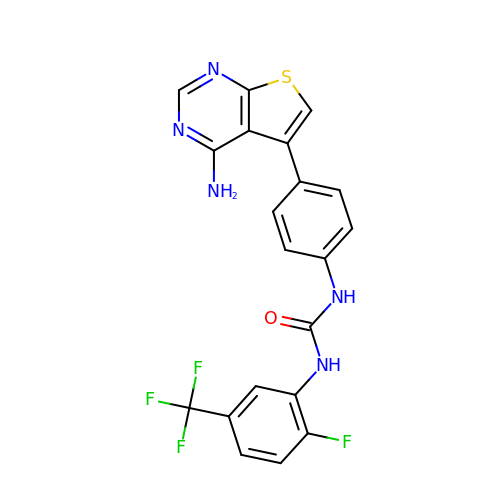1-[4-(4-aminothieno[2,3-d]pyrimidin-5-yl)phenyl]-3-[2-fluoro-5-(trifluoromethyl)phenyl]urea | C20 H13 F4 N5 O S | PTVPBWWDGZSEAF-UHFFFAOYSA-N>RTKIVVKVHMPCDKSRAKAMALAASVNGVDVVEITGEDKDRLVVVGRGIDPVRLVALLREKCGLAELLMVELV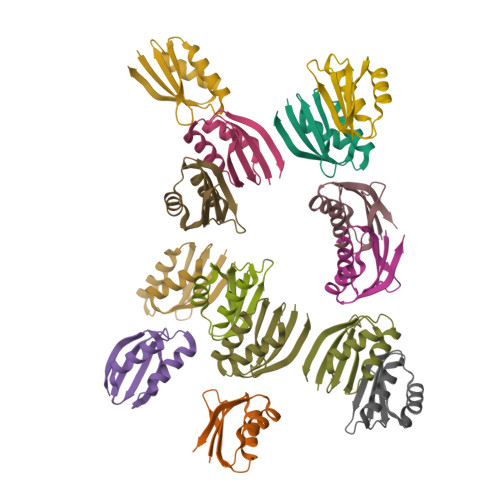[14x]>SNAMAKVKIVGILNVTPNSFHDGGRFVETDKAVVRARELLSQGADIIEIGGESTGPGSNTITADEELARIVPVIRAIRSSLPDANIAVDTYKAEVARKALELGATMINDVSAGRADPKLFGVVARSNAQIVLMYSKDTDPHTSFDERQYVDVVRTVYDFLAERKKAAMSAGIPADRIILDTGLGHFVSSDPQYSFQLLAHLSDFQDLGCKLFLSPSRKSFLAGNELLKTADRLPGTIAASAIAVLHGADYIRTHDVLEVRRGCEIATAINQP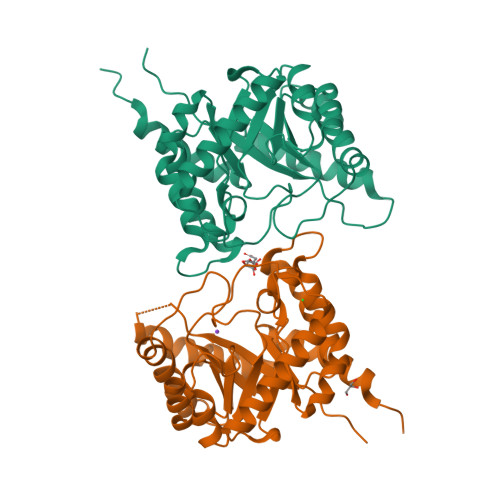PER[2x]pmcMechanistic target of rapamycin (mTOR, also known as mammalian TOR) is an essential serine/threonine protein kinase that responds to nutrients, growth factors, and cellular energy to promote cell growth. mTOR nucleates two distinct complexes, mTORC1 and mTORC2, each characterized by specific subunits, targets, downstream signaling pathways, and functions. mTORC1 contains mTOR, regulatory-associated protein of mTOR (RAPTOR), and mammalian lethal with SEC13 protein 8 (mLST8). RAPTOR binds mTORC1 substrates, including the well-characterized substrates ribosomal protein S6 kinase 1 (S6K1) and 4E binding protein 1 (4E-BP1), through a five-amino acid motif termed TOS. RAPTOR binds the LST2 TOS sequence to present LST2 to the kinase catalytic site in mTOR for phosphorylation of LST2 S670. mTORC1-dependent phosphorylation at S670 leads to monoubiquitination and stabilization of LST2.

To further improve the resolution of the visualization of TOS motif interactions, we analyzed mTORC1 in complex with the synthetic LST2 TOS peptide, for which higher concentrations could be reached compared to full-length LST2. Single-particle cryo-EM analysis achieved a resolution of 3.27 Å (map6—SI Appendix) for the TOS-binding RAPTOR region. This allowed atomic modeling of nine peptide residues (corresponding to amino acids 399 to 407 in full-length LST2), including the TOS motif, in the RAPTOR TOS-binding pocket. The LST2 TOS peptide contains three negatively charged residues which make electrostatic interactions with the positively charged TOS-binding pocket. F401 and M403 anchor the TOS peptide by binding in particularly deep cavities in the TOS-binding site, via hydrophobic interactions with surrounding residues. Finally, a comparison of LST2 TOS and previously described 4E-BP1 TOS binding shows that the TOS peptides, in particular, the consensus phenylalanine (F401 in LST2 and F114 in 4E-BP1), share a common mode of binding to the RAPTOR pocket. Superimposition of the two TOS peptides in the RAPTOR binding pocket shows that the first phenylalanine of the TOS motif lies in the same position in both structures. The TOS peptide bound RAPTOR with a dissociation constant (Kd) of 330 nM. The TOS–RAPTOR interaction was abrogated by a single residue replacement in the TOS peptide equivalent to a F401A point mutation.

> HHHHHHHHHHEQKLISEEDLDYKDDDDKMESEMLQSPLLGLGEEDEADLTDWNLPLAFMKKRHCEKIEGSKSLAQSWRMKDRMKTVSVALVLCLNVGVDPPDVVKTTPCARLECWIDPLSMGPQKALETIGANLQKQYENWQPRARYKQSLDPTVDEVKKLCTSLRRNAKEERVLFHYNGHGVPRPTVNGEVWVFNKNYTQYIPLSIYDLQTWMGSPSIFVYDCSNAGLIVKSFKQFALQREQELEVAAINPNHPLAQMPLPPSMKNCIQLAACEATELLPMIPDLPADLFTSCLTTPIKIALRWFCMQKCVSLVPGVTLDLIEKIPGRLNDRRTPLGELNWIFTAITDTIAWNVLPRDLFQKLFRQDLLVASLFRNFLLAERIMRSYNCTPVSSPRLPPTYMHAMWQAWDLAVDICLSQLPTIIEEGTAFRHSPFFAEQLTAFQVWLTMGVENRNPPEQLPIVLQVLLSQVHRLRALDLLGRFLDLGPWAVSLALSVGIFPYVLKLLQSSARELRPLLVFIWAKILAVDSSCQADLVKDNGHKYFLSVLADPYMPAEHRTMTAFILAVIVNSYHTGQEACLQGNLIAICLEQLNDPHPLLRQWVAICLGRIWQNFDSARWCGVRDSAHEKLYSLLSDPIPEVRCAAVFALGTFVGNSAERTDHSTTIDHNVAMMLAQLVSDGSPMVRKELVVALSHLVVQYESNFCTVALQFIEEEKNYALPSPATTEGGSLTPVRDSPCTPRLRSVSSYGNIRAVATARSLNKSLQNLSLTEESGGAVAFSPGNLSTSSSASSTLGSPENEEHILSFETIDKMRRASSYSSLNSLIGVSFNSVYTQIWRVLLHLAADPYPEVSDVAMKVLNSIAYKATVNARPQRVLDTSSLTQSAPASPTNKGVHIHQAGGSPPASSTSSSSLTNDVAKQPVSRDLPSGRPGTTGPAGAQYTPHSHQFPRTRKMFDKGPEQTADDADDAAGHKSFISATVQTGFCDWSARYFAQPVMKIPEEHDLESQIRKEREWRFLRNSRVRRQAQQVIQKGITRLDDQIFLNRNPGVPSVVKFHPFTPCIAVADKDSICFWDWEKGEKLDYFHNGNPRYTRVTAMEYLNGQDCSLLLTATDDGAIRVWKNFADLEKNPEMVTAWQGLSDMLPTTRGAGMVVDWEQETGLLMSSGDVRIVRIWDTDREMKVQDIPTGADSCVTSLSCDSHRSLIVAGLGDGSIRVYDRRMALSECRVMTYREHTAWVVKASLQKRPDGHIVSVSVNGDVRIFDPRMPESVNVLQIVKGLTALDIHPQADLIACGSVNQFTAIYNSSGELINNIKYYDGFMGQRVGAISCLAFHPHWPHLAVGSNDYYISVYSVEKRVR;> DEEERVFFMDDVE> MAQRKNAKSSGNSSSSGSGSGSTSAGSSSPGARRETKHGGHKNGRKGGLSGTSFFTWFMVIALLGVWTSVAVVWFDLVDYEEVLGKLGIYDADGDGDFDVDDAKVLLGLKERSTSEPAVPPEEAEPHTEPEEQVPVEAEPQNIEDEAKEQIQSL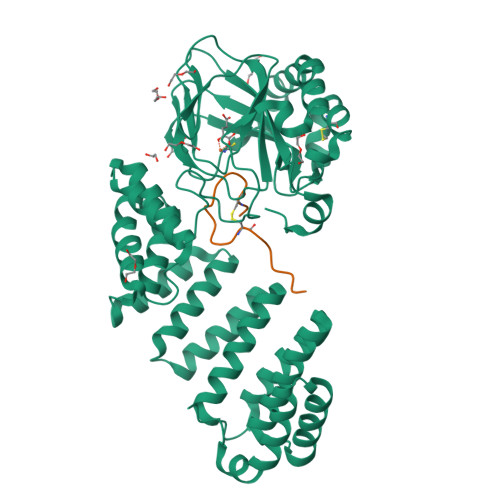LHEMVHAEHVEGEDLQQEDGPTGEPQQEDDEFLMATDVDDRFETLEPEVSHEETEHSYHVEETVSQDCNQDMEEMMSEQENPDSSEPVVEDERLHHDTDDVTYQVYEEQAVYEPLENEGIEITEVTAPPEDNPVEDSQVIVEEVSIFPVEEQQEVPPETNRKTDDPEQKAKVKKKKPKLLNKFDKTIKAELDAAEKLRKRGKIEEAVNAFKELVRKYPQSPRARYGKAQCEDDLAEKRRSNEVLRGAIETYQEVASLPDVPADLLKLSLKRRSDRQQFLGHMRGSLLTLQRLVQLFPNDTSLKNDLGVGYLLIGDNDNAKKVYEEVLSVTPNDGFAKVHYGFILKAQNKIAESIPYLKEGIESGDPGTDDGRFYFHLGDAMQRVGNKEAYKWYELGHKRGHFASVWQRSLYNVNGLKAQPWWTPKETGYTELVKSLERNWKLIRDEGLAVMDKAKGLFLPEDENLREKGDWSQFTLWQQGRRNENACKGAPKTCTLLEKFPETTGCRRGQIKYSIMHPGTHVWPHTGPTNCRLRMHLGLVIPKEGCKIRCANETKTWEEGKVLIFDDSFEHEVWQDASSFRLIFIVDVWHPELTPQQRRSLPAI;> DGDQSETSPSQNQGKCKNGLGEYTCTSLEGFEGKNSELF>[2x]MKILRGEEIAEKKAENLHGIIERSGLEPSLKLIQIGDNEAASIYARAKIRRGKKIGIAVDLEKYDDISMKDLLKRIDDLAKDPQINGIMIENPLPKGFDYYEIVRNIPYYKDVDALSPYNQGLIALNREFLVPATPRAVIDIMDYYGYHENTVTIVNRSPVVGRPLSMMLLNRNYT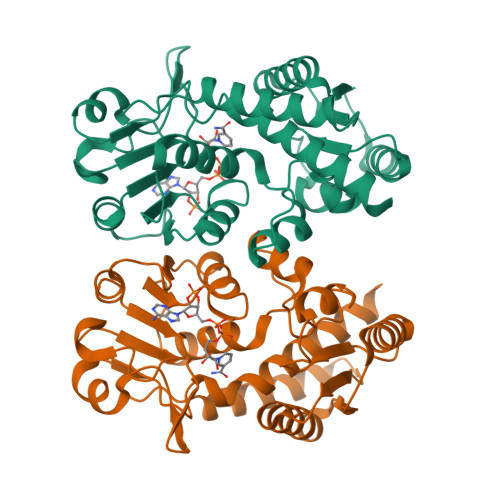VSVCHSKTKDIGSMTRSSKIVVVAVGRPGFLNREMVTPGSVVIDVGINYVNDKVVGDANFEDLSEYVEAITPVPGGVGPITATNILENVVKAAEFQKNNL> GSTQAAPFPELCSYTWEAVDTKNNVLYKINICGSVDIVQCGPSSAVCMHDLKTRTYHSVGDSVLRSATRSLLEFNTTVSCDQQGTNHRVQSSIAFLCGKTLGTPEFVTATECVHYFEWRTTAACKKDIFKANKEVPCYVFDEELRKHDLNPLIKLSGAYLVDDSDPDTSLFINVCRDIDTLRDPGSQLRACPPGTAACLVRGHQAFDVGQPRDGLKLVRKDRLVLSYVREEAGKLDFCDGHSPAVTITFVCPSERREGTIPKLTAKSNCRYEIEWITEYACHRDYLESKTCSLSGEQQDVSIDLTPLAQSGGSSYISDGKEYLFYLNVCGETEIQFCNKKQAAVCQVKKSDTSQVKAAGRYHNQTLRYSDGDLTLIYFGGDECSSGFQRMSVINFECNKTAGNDGKGTPVFTGEVDCTYFFTWDTEYACVKEKEDLLCGATDGKKRYDLSALVRHAEPEQNWEAVDGSQTETEKKHFFINICHRVLQEGKARGCPEDAAVCAVDKNGSKNLGKFISSPMKEKGNIQLSYSDGDDCGHGKKIKTNITLVCKPGDLESAPVLRTSGEGGCFYEFEWHTAAACVLSKTEGENCTVFDSQAGFSFDLSPLTKKNGAYKVETKKYDFYINVCGPVSVSPCQPDSGACQVAKSDEKTWNLGLSNAKLSYYDGMIQLNYRGGTPYNNERHTPRATLITFLCDRDAGVGFPEYQEEDNSTYNFRWYTSYACPEEALVPR

Delivery of these newly synthesized hydrolytic enzymes to lysosomes depends on the P-type lectins, 300-kDa cation-independent mannose 6-phosphate receptor (CI-MPR) and 46-kDa cation-dependent MPR (CD-MPR), that bind the carbohydrate determinant, mannose 6-phosphate (M6P), on lysosomal enzymes. CI-MPR’s extracytoplasmic region contains 15 homologous domains called “mannose 6-phosphate receptor homology” domains (MRH) due to their similar size (~150 residues) and conserved residues, including disulfide bonding. CI-MPR has four non-adjacent CRDs (domains 3, 5, 9, and 15), each with distinctive phosphomonoester and phosphodiester glycan preferences. We now report the crystal structures of the N-terminal five domains of human CI-MPR, revealing the orientation of two CRDs (domains 3 and 5) with respect to each other at pH 5.5 and 7.0.

Crystallization screening of human CI-MPR domains 1–5 protein in the presence of 10-mM M6P resulted in two conditions yielding diffraction quality crystals. Interestingly, both conditions show evidence of the N-glycan at N591 of a crystallographic neighbor partially occupying the carbohydrate-binding site of domain 5. The pH 5.5 structure had sufficient occupancy to allow carbohydrate refinement while the corresponding region in the pH 7.0 structure did not. The other CRD (domain 3) remains unoccupied in both structures, unlike bovine CI-MPR domains 1–3, where we showed domain 3 was bound to a ligand: either M6P or the oligosaccharide of a crystallographic neighbor (inset). Although we were surprised that the domain-3 binding pocket did not contain M6P at pH 7.0 conditions, the presence of the N-linked glycan near the binding site of domain 5 could perturb conformational equilibria between substructures that stabilize a domain arrangement most favorable for crystallographic packing. The interdomain linker between domains 2 and 3 adopts a more extended structure in the absence of ligand, allowing for the repositioning of domain 3. In the absence of a ligand bound to domain 3, its C-terminal face contacts the C-terminal face of domain 1. The flexibility of domain 4 was also recently demonstrated in the cryo-EM structures published by Wang et al. at the time of this paper’s submission. Comparing their bovine domains 4–14 structure at pH 7.4 in the presence of IGF2 with our human domains 1–5 structure at pH 5.5 or 7.0 shows domain 4 rotated ~180°. Another possibility is that PPT1 binding to domain 3 causes a rearrangement of domains such that the binding site of domain 5 is no longer accessible by ligand. This latter possibility of allosteric interactions between the CRDs is consistent with our crystal structures that illustrate that domain interactions can be dramatically altered in the presence or absence of ligands, such as between domain 3 and domains 1 and 2.>[3x]GSHMESLTQYIPDEFSMLRFGKKFAEILLKLHTEKAIMVYLNGDLGAGKTTLT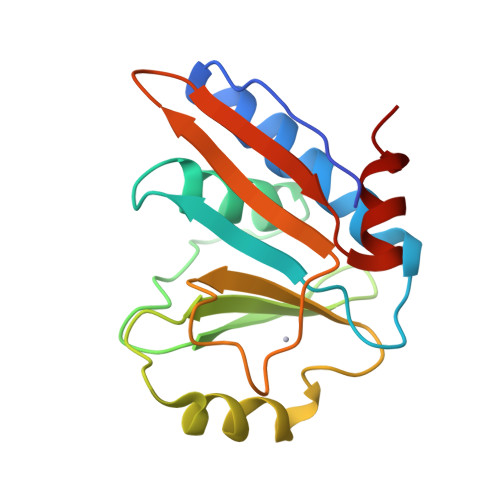RGMLQGIGHQGNVKSPTYTLVEEYNIAGKMIYHFDLYRLADPEELEFMGIRDYFNTDSICLIEWSEKGQGILPEADILVNIDYYDDARNIELIAQTNLGKNIISAFSN4-[[(6-bromanyl-1~{H}-indazol-4-yl)amino]methyl]phenol | C14 H12 Br N3 O | 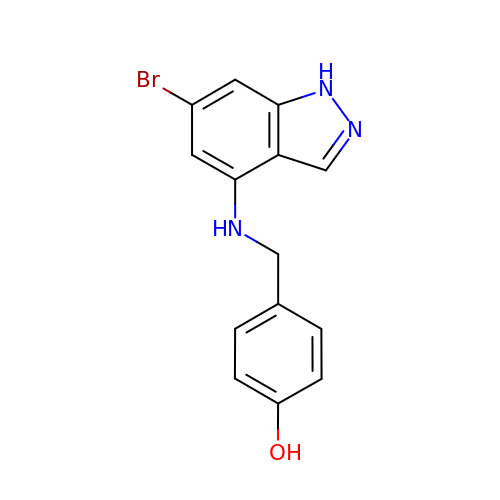YLKYPFSLPHIKQR-UHFFFAOYSA-N> HLVCPMSKSPYVDPHKSGHEIWEEFSMSFTPAVKEVVEFAKRIPGFRDLSQHDQVNLLKA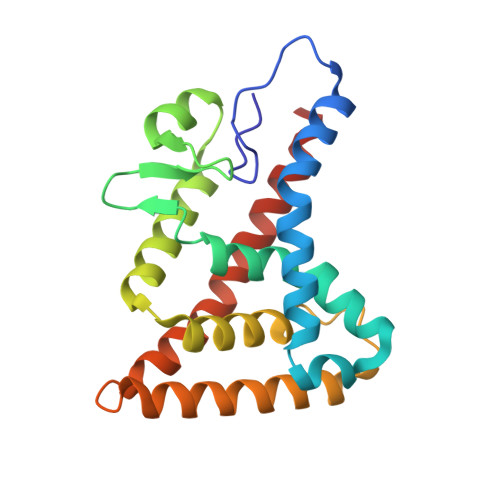GTFEVLMVRFASLFDAKERTVTFLSGKKYSVDDLHSMGAGDLLNSMFEFSEKLNALQLSDEEMSLFTAVVLVSADRSGIENVNSVEALQETLIRALRTLIMKNHPNEASIFTKLLLKLPDLRSLNNMHSEELLAFKVHP> MKLEINKFNYNDPIDGINVITMRPPRHSDKINKGKGPFKAFQVIKNIWIVPERYNFTNNTNDLNIPSEPIMEADAIYNPNYLNTPSEKDEFLQGVIKVLERIKSKPEGEKLLELISSSIPLPL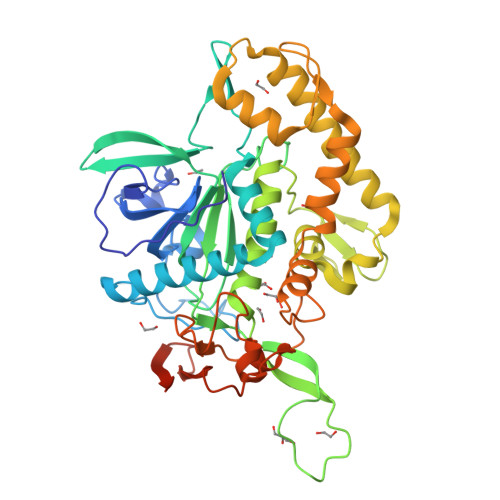VSNGALTLSDNETIAYQENDNIVSTLQANLVIYGPGPDIANNEIYGLYSTPISNGEGTLSEVSFSPFYLKPFDESYGNYRSLVNIVNKFVKREFAPDPASTLMHELVHVTHNLYGISNRNFYYNFDTGKIETSRQQNSLIFEELLTFGGIDSKAISSLIIKKIIETAKNNYTTLISERLNTVTVENDLLKNIKNKIPVQGRLGNFKLDTAEFEKKLNTILFVLNESNLAQRFSILVRKHYIKERPIDPIYVNILDDNSYSTLEGFNISSQGSNDFQGQLLESSYFEKIESNALRAFIKICPRNGLLYNAIYRNSKNHHHHHH>[2x]CGAG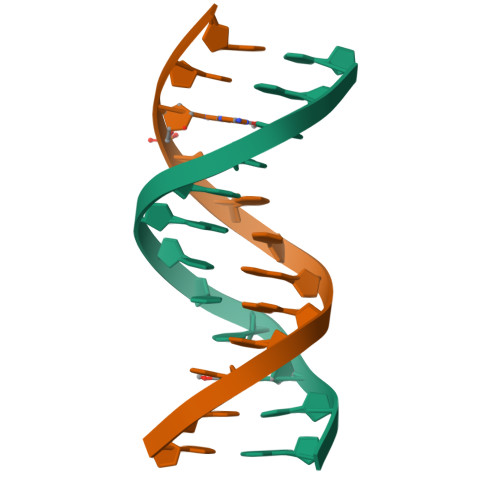AATTCGCG> VDCSEYPKPACTKEYR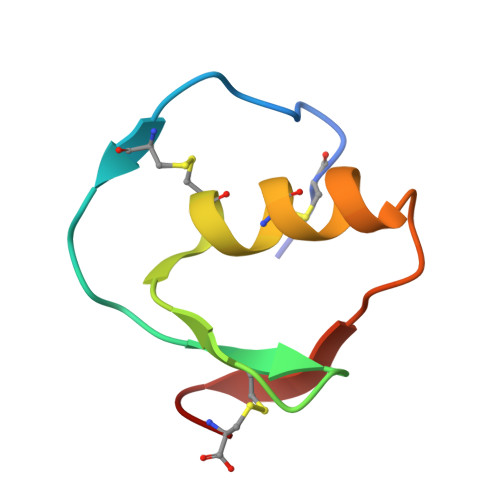PLCGSDNKTYGNKCNFCNAVVESNGTLTLSHFGKC> MASPRANDAPIVLLHGFTGWGREEMLGFKYWGGVRGDIEQWLNDNGYRTYTLAVGPLSSNWDRACEAYAQLVGGTVDYGAAHAAKHGHARFGRTYPGLLPELKRGGRVHIIAHSQGGQTARMLVSLLENGSQEEREYAKAHNVSLSPLFEGGHHFVLSVTTIATPHDGTTLVNMVDF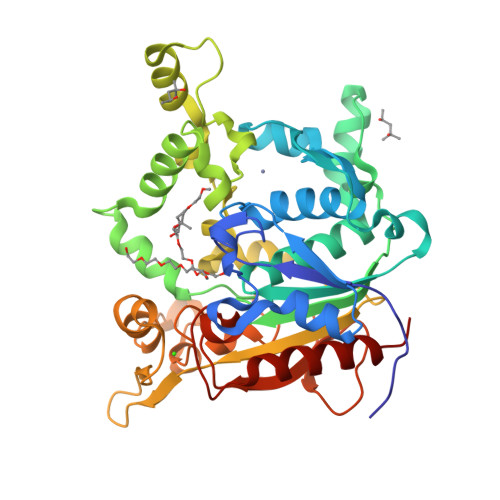TDRFFDLQKAVLKAAAVASNVPYTSQVYDFKLDQWGLRRQPGESFDHYFERLKRSPVWTSTDTARYDLSIPGAEKLNQWVQASPNTYYLSFSTERTHRGALTGNYYPELGMNAFSAVVCAPFLGSYRNEALGIDDRWLENDGIVNTVSMNGPKRGSSDRIVPYDGTLKKGVWNDMGTYNVDHLEVIGVDPNPSFDIRAFYLRLAEQLASLRP>[2x]NTKYNKEFLLYLAGFVDGDGSIIAQIKPNQSYKFKHQLSLTFQVTQKTQRRWF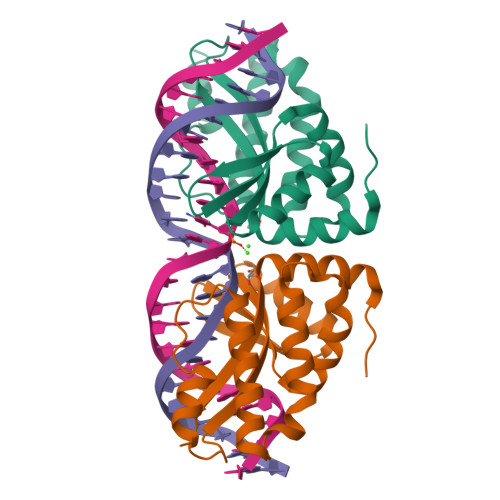LDKLVDEIGVGYVRDRGSVSDYILSEIKPLHNFLTQLQPFLKLKQKQANLVLKIIEQLPSAKESPDKFLEVCTWVDQIAALNDSKTRKTTSETVRAVLD> GMQMELQSPEYKLSKLRTSTIMTDYNPNYCFAGKTSSISDLKEVPRKNITLIRGLGHGAFGEVYEGQVSGMPNDPSPLQVAVKTLPEVCSEQDELDFLMEALIISKFNHQNIVRCIGVSLQSLPRFILMELMAGRDLKSFLRETRPRPSQPSSLAMLDLLHVARDIACGCQYLEENHFIHRDIAARNCLLTCPGPGRVAKIGDFGMARDIYRASYYRK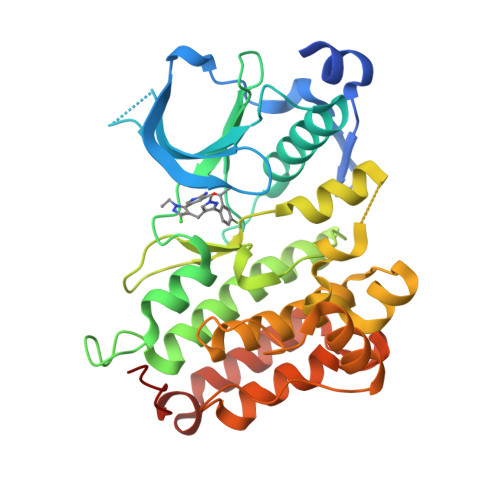GGCAMLPVKWMPPEAFMEGIFTSKTDTWSFGVLLWEIFSLGYMPYPSKSNQEVLEFVTSGGRMDPPKNCPGPVYRIMTQCWQHQPEDRPNFAIILERIEYCTQDPDVINTALPIEYGPLVEEEEKV> GNNNSTKESTHDNHSDSSTH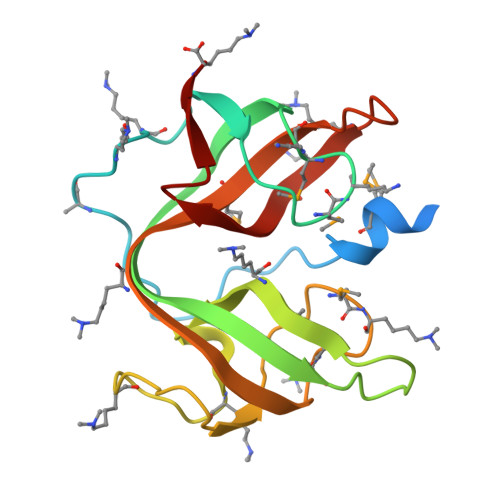EEMDHSGSADVPEGLQESKNPKYKVGSQVIINTSHMKGMKGAEATVTGAYDTTAYVVSYTPTNGGQRVDHHKWVIQEEIKDAGDKTLQPGDQVILEASHMKGMKGATAEIDSAEKTTVYMVDYTSTTSGEKVKNHKWVTEDELSAK> SLFELGKMIWQETGKNPVKNYGLYGCNCGVGGRGEPLDATDRCCFVHKCCYKKLTDCDSKKDRYSYKWKNKAIVCGKNQPCMQEMCECDKAFAICLRENLDTYNKSFRYHL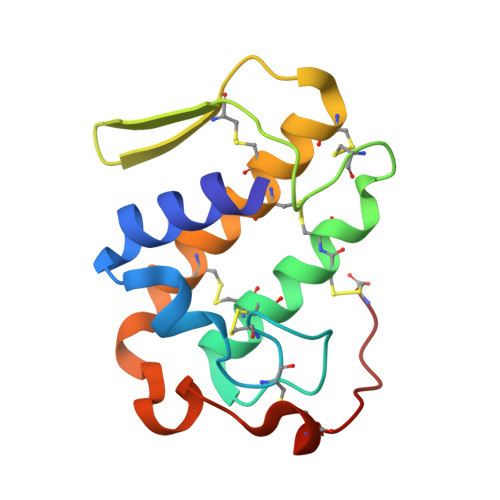KPSCKKTSEQC> PPGPE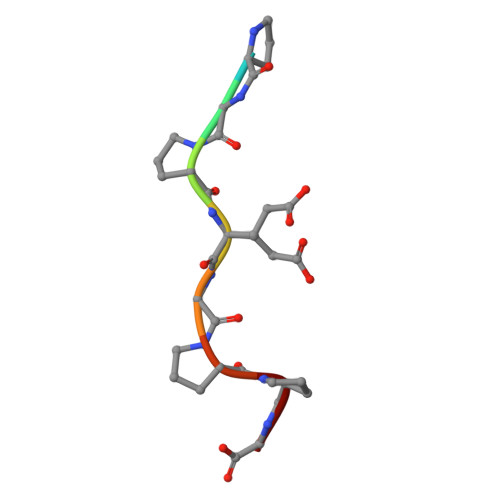GPPG[(3S)-3,7-dimethyloct-6-enyl] phosphono hydrogen phosphate | C10 H22 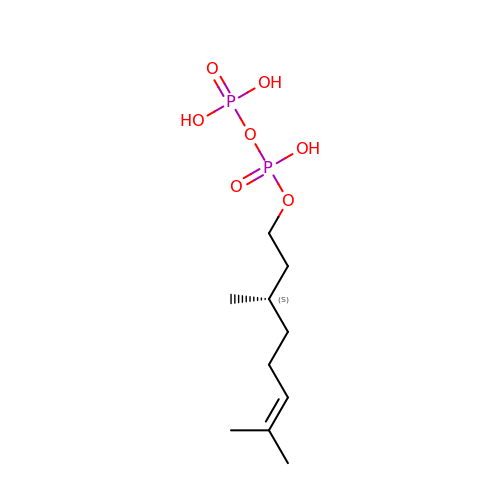O7 P2 | MDPFRHMROKBMSH-JTQLQIEISA-N>[2x]GPMLADLDHFGKNYKHDEEAQRNQKPWMLTWPQIKLVLLAGVGFFLDAYDLFIINQVAPMLAQVYFPKTGLPAQRQDLMKAAANIGCVVGQVMFGV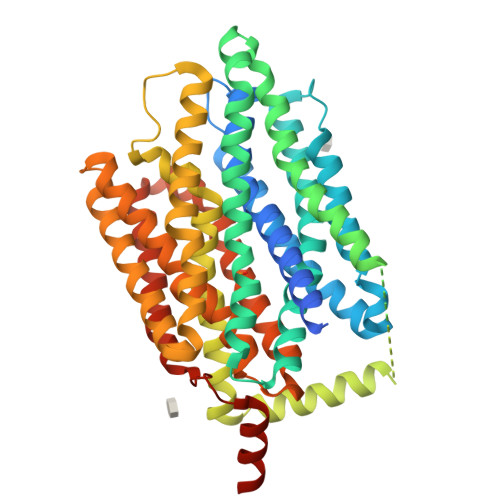LGDSFGRKFVYGKELILIIVATIFQMSAPSHWDGNRVLTWITICRVFLGIGIGGDYPMSATVVSDRANIHRRGTLLCFIFANQGWGSFVGSLVTIVTISGFKHRLKSGHTHDVDKAWRILIGLSLIPAFGTLYQRLTLPESRKFELTRDAASSSTVAIDKKDHDATHEVKDAPESEKSSPKVTPADAIDDDRHGVIASKKAHWQEFVAYFSTWNHFRNLLGSMLGWFLVDIAFYGINLNQSVVLAQIGFAGKTGDVYDKLFQLATGNIIVTALGFLPGYYFTLFLIDIVGRKKLQFMGFIMSGLFLAILAGEIDHIGKGPLLACFTFMQFFFNFGANTTTFIVAAELFPTRIRASAHGISAAAGQCGAILSSLVFNQLKAKIGTSAVLWIFFSTCILGFISTFLIDETMGVDPDEKDLEERRARGEIPGGLVPR>SELRDRQAIFETLVAKGRELLACDRVIVYAFDDNYVGTVVAESVAEGWPQARDQVIEDPCFREHWVEAYRQGRIQATTDIFKAGLTECHLNQLRPLKVRANLVVPMVIDDQLFGLLIAHQAS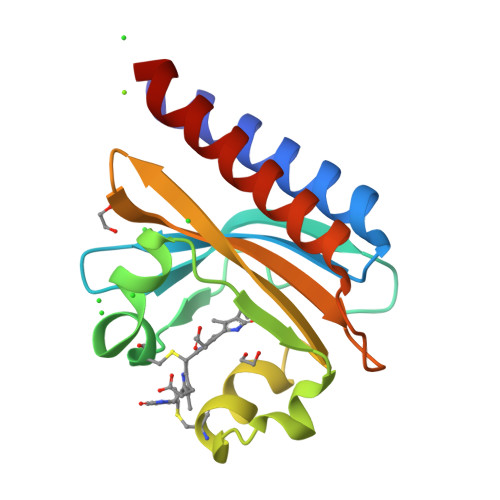EPRQWQEIEIDQFSELASTGSLVLERLH[2x]> MGPVWRKHYITYRINNYTPDMNREDVDYAIRKAFQVWSNVTPLKFSKINTGMADILVVFARGAHGDDHAFDGKGGILAHAFGPGSGIGGDAHFDEDEFWT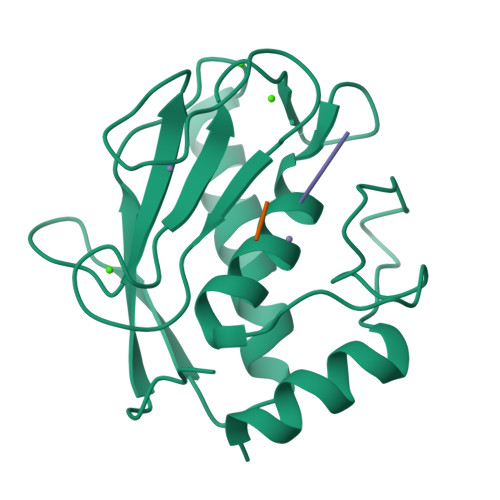THSGGTNLFLTAVHEIGHSLGLGHSSDPKAVMFPTYKYVDINTFRLSADDIRGIQSLYG;> IAG;> PQG>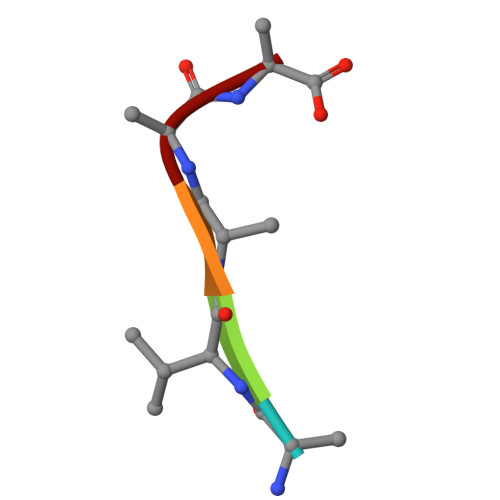 RVAAA The sixth gene of the tdc operon encodes a protein, TdcF, that is a member of the YjgF/YER057c/UK114 family. The location of this gene within the tdc operon is strongly suggestive of a role in the degradation of 2-ketobutyrate. Each 14 kDa subunit comprises a single domain that contains a predominantly anti-parallel, six-stranded β-sheet against which are packed two short α-helices. The most significant structural features are the three symmetry-related solvent-accessible clefts, located at the interfaces between pair of subunits, close to the "equator" of the trimer.

A further data set was collected to 1.6 Å resolution, this time from a crystal soaked in 1 mM ketobutyrate. The resultant electron density maps showed clear density for a 2-ketobutyrate ligand in each of the three binding sites. As with the serine ligand, the carboxylate moiety of 2-ketobutyrate makes a bi-dentate salt-bridge to the side-chain of Arg-105, whilst the keto group forms two hydrogen bonds, one with the amino group of Cys-107, and the other with the carboxyl group of Glu-120. However, in order to provide a hydrogen for the latter interaction, the ligand would need to bind in the less stable enol form. Curiously, there is a water molecule adjacent to the 2-ketobutyrate on the re-face of the enol moiety and approximately 2.8 Å from C2. The observation of a water molecule stacked against one face of the enol moiety of the 2-ketobutyrate is intriguing as it could take part in catalysis. By contrast, full site occupancy was achieved using 2-ketobutyrate, indicating that it binds with higher affinity than the other ligands. A comparison of the four TdcF structures presented here shows that the largest changes occur between the 1.6 Å resolution structures of the as-isolated and the 2-ketobutyrate-bound forms. A further modification was apparent at Lys-58 in just the A chain of the 2-ketobutyrate-bound structure. This was modelled as a carboxylated lysine in two alternative conformations.

>MKKIIETQRAPGAIGPYVQGVDLGSMVFTSGQIPVCPQTGEIPADVQDQARLSLENVKAIVVAAGLSVGDIIKMTVFITDLNDFATINEVYKQFFDEHQATYPTRSCVQVARLPKDVKLEIEAIAVRSA[3x]(4R)-4-[(1R)-1-{[6-(3,4-dimethoxyphenyl)[1,3]thiazolo[5,4-c]pyridin-4-yl]oxy}ethyl]pyrrolidin-2-one | C20 H21 N3 O4 S | 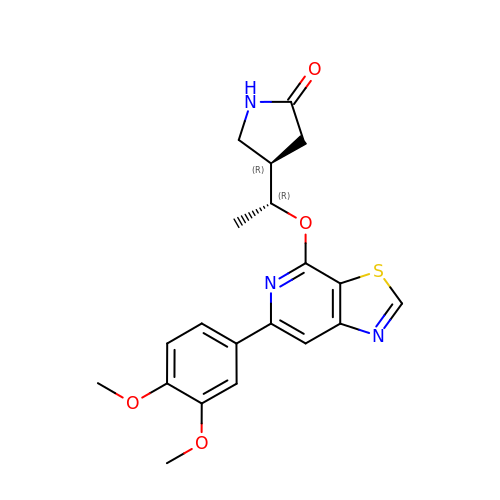OTUKQYFHRKKGEI-DGCLKSJQSA-N>MEGGGKPNSSSNSRDDGNSVFPAKASATGAGPAAAEKRLGTPPGGGGAGAKEHGNSVCFKVDGGGGGGGGGGGGEEPAGGFEDAEGPRRQYGFMQRQFTSMLQPGVNKFSLRMFGSQKAVEKEQERVKTAGFWIIHPYSDFRFYWDLIMLIMMVGNLVIIPVGITFFTEQTTTPWIIFNVASDTVCLLDLIMNFRTGTVNEDSSEIILDPKVIKMNYLKSWFVVDFISSIPVDYIFLIVEKGMDSEVYKTARALRIVRFTKILCLLRLLRLSRLIRYIHQWEEIFHMTYDLASAVVRIFNLIGMMLLLCHWDGCLQFLVPLLQDFPPDCWVSLNEMVNDSWGKQYSYALFKAMSHMLCIGYGAQAPVSMSDLWITMLSMIVGATCYAMFVGHATALIQSLDSSRRQYQEKYKQVEQYMSFHKLPADMRQKIHDYYEHRYQGKIFDEENILNELNDPLREEIVNFNCRKLVATMPLFANADPNFVTAMLSKLRFEVFQPGDYIIREGAVG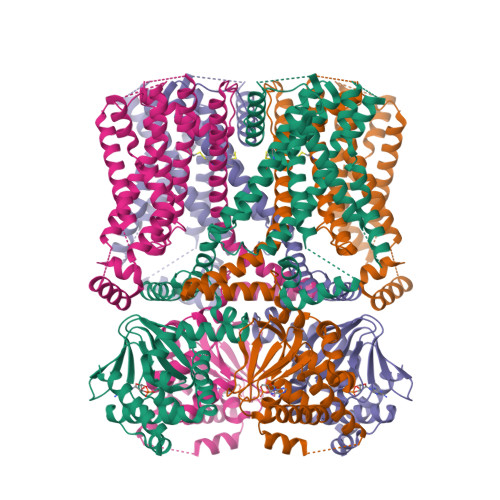KKMYFIQHGVAGVITKSSKEMKLTDGSYFGEICLLTKGRRTASVRADTYCRLYSLSVDNFNEVLEEYPMMRRAFETVAIDRLDRIGKKNSILLQKFQKDLNTGVFNNQENEILKQIVKHDREMVQAIAPINYPQMTTLNSTSSTTTPTSRMRTQSPPVYTATSLSHSNLHSPSPSTQTPQPSAILSPCSYTTAVCSPPVQSPLAARTFHYASPTASQLSLMQQQPQQQVQQSQPPQTQPQQPSPQPQTPGSSTPKNEVHKSTQALHNTNLTREVRPLSASQPSLPHEVSTLISRPHPTVGESLASIPQPVTAVPGTGLQAGGRSTVPQRVTLFRQMSSGAIPPNRGVPPAPPPPAAALPRESSSVLNTDPDAEKPRFASNL[4x]> QDNSRYTHFLTQHYDAKPQGRDDRYCESIMRRRGLTSPCKDINTFIHGNKRSIKAICENKNGNPHRENLRISKSSFQVTTCKLHGGSPWPPCQY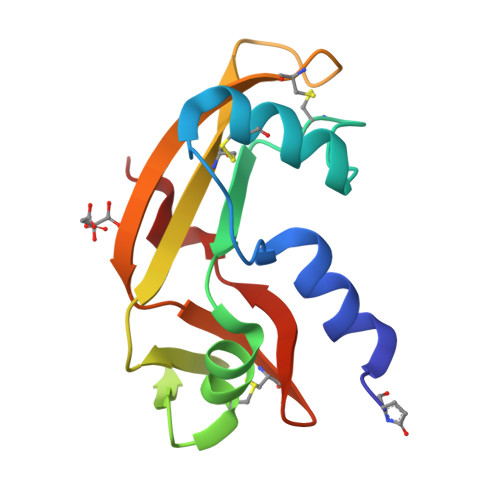RATAGFRNVVVACENGLPVHLDGSIFRRP> GCQSNHILKHNRCKQDSDCLAGC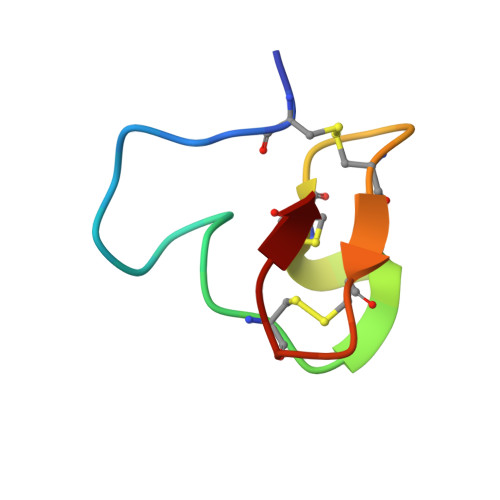VCGPNGFCG>AMKDLKGTKTAENLKQGFIGESMANRRYLYFAKRADEEGYPEIAGLLRSIAEGETAHAFGHLDFIRQGGLTDPATDKPIGTLEQMIESAIAGETYEWTQMYPGFAKVAREEGFPEVAEWFETLARAEKSHAEKFQNVLKQLKGGT[2x]

One such protein is sulerythrin (SulE), a ruberythrin-like protein isolated from the thermophilic archeon Sulfolobus tokodaii. SulE lacks the characteristic C-terminal, rubredoxin-like FeS4 domain of ruberythrins and contains a binuclear metal centre that coordinates iron and zinc when isolated from S. tokodaii. In contrast to other members of the ruberythrin family, a crystal structure of native SulE shows that it forms homodimers through domain swapping, with each monomer contributing two α-helices to give two four-helix bundles that each harbour a solvent-accessible, single dimetal site. The exact function of SulE is unknown, but it is presumed to be involved in reactions against oxidative stress.

Diffraction data from a crystal of recombinantly expressed SulE reconstituted with iron (diFe-SulE) were collected on beamline BL14.1 at the BESSY II electron-storage ring operated by the Helmholtz-Zentrum Berlin (HZB). The beamline flux was set to 5% to minimize radiation-induced damage to the metal centres for initial characterization. The crystal diffracted to 1.42 Å resolution and belonged to space group P63. The edges for Fe-2 and Fe-4 are shifted to higher energies by 2 eV compared with Fe-1 and Fe-3. This indicates that Fe-2 and Fe-4 are in a more oxidized state than Fe-1 and Fe-3 and are likely to be ferric irons, based on the observation that an increase in oxidation leads to an edge shift of between 1 and 5 eV in model iron compounds.> GPLGSMDEDVLPGEVLAIEGIFMACGLNEPEYLYHPLLSPIKLYITG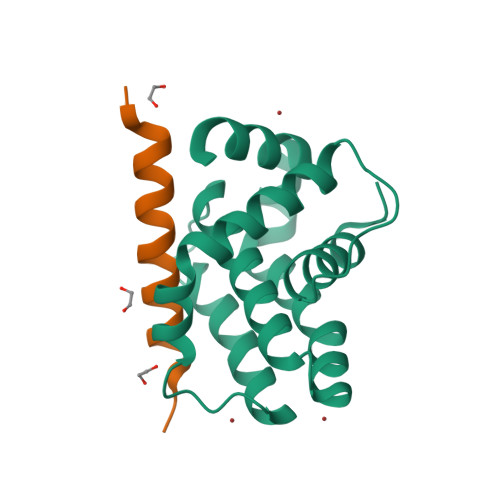LMRDKESLFEAMLANVRFHSTTGINQLGLSMLQVSGDGNMNWGRALAILTFGSFVAQKLSNEPHLRDFALAVLPAYAYEAIGPQWFRARGGWRGLKAYCTQVLT;> EEQWAREIGAQLRRMADDLNAQYERR>GPGSSLSRFRGCLAGALLGDCVGSFYAAHDTVDLTSVLRHVQSLEPDPGTPGSERTEALYYTDDTAMARALVQSLLAKEAFDEVDMAHRFAQEYKKDPDRGYGAGVVTVFKKLLNPKCRDVFEPARAQFNGKGSYGNGGAMRVAGISLAYSSVQDVQKFARLSAQLTHASSLGYNGAILQALAVHLALQGESSSEHFLKQLLGHMEDLEGDAQSVLDARELGMEERPYSSRLKKIGELLDQASVTREEVVSELGNGIAAFESVPTAIYCFLRCMEPDPEIPSAFNSLQRTLIYSISLGGDTDTIATMAGAIAGAYYGMDQVPESWQQSCEGYEETDILAQSLHRVFQKS[2x]

Poly(ADP-ribose)glycohydrolase (PARG) and (ADP-ribosyl)hydrolase 3 (ARH3) are the main hydrolases of serine PAR- and MARylation, respectively, thus playing a pivotal role in signal silencing following DNA damage. ARH3 is the only known enzyme to reverse serine MARylation and is consequently responsible for the regulation of hundreds of ADP-ribosylated proteins following DNA damage. In contrast to PARG, the active site of ARH3 contains a catalytic binuclear magnesium centre. To understand the impact of the ARH3:substrate interaction on reaction efficiency, we crystallised ARH3 in complex with the chemically synthesised substrates: histone H2B peptide (aa 1–11) MARylated on Ser7 (H2BS7mar), dimeric ADP-ribose (dimer) and α-NAD+.

Therefore, we chose to crystallise the hARH3 E41A substrate complexes as this prevents substrate cleavage during crystal formation, while retaining a functionally relevant magnesium coordination. Our structural data further reveal that in the α-NAD+ complex Glu41 would be displaced from the axial MgII position by the nicotinamide moiety, thus forcing the observed open conformation. Within the hARH3:α-NAD+ complex, the interaction between nicotinamide and MgII is sterically dominated by the binding of the ADPr moiety within the active site. The positive charge at the N1 nitrogen and long MgII-ring atom distances (3.4–4.1 Å) suggest that the arene cannot act like a chelant to displace MgII from the protein coordination. However, the nicotinamide moiety sterically prevents occupation of the axial ligand position of MgII, thus creating a free valence at the Mg2+ ion and forcing the Glu41-flap to open. In addition, the nicotinamide positioning is distinctly asymmetric, reminiscent of ring slippage, which may polarise the π electron system and weaken the N-glycosidic bond. Noteworthy, neither the H2BS7mar nor the α-NAD+ complex have a water ligand at MgII, thus excluding the ion as a water activator during the reaction cycle. The relative distance between magnesium ion and nicotinamide in our structure suggests that rather than engaging in metal coordination, the ligand displacement leads to a free valence and a high energy magnesium state. Together with slippage-like positioning of the nicotinamide ring, which introduced polarisation into the π electron system, it likely provides the energy for bond cleavage.>GSELRSIAFSRAVFAEFLATLLFVFFGLGSALNWPQALPSVLQIAMAFGLGIGTLVQALGHISGAHINPAVTVACLVGCHVSVLRAAFYVAAQLLGAVAGAALLHEITPADIRGDLAVNALSNSMTAGQAVTVELFLTLQLVLCIFASTDERRGENPGTPALSIGFSVALGHLLGIHYTGCSMNPARSLAPAVVTGKFDDHWVFWIGPLVGAILGSLLYNYVLFPPAKSLSERLAVLKGLE[4x]

Aquaporins are water channels found in the cell membrane, where they allow the passage of water molecules in and out of the cells. In the kidney collecting duct, arginine vasopressin-dependent trafficking of aquaporin-2 (AQP2) fine-tunes reabsorption of water from pre-urine, allowing precise regulation of the final urine volume. Point mutations in the gene for AQP2 may disturb this process and lead to nephrogenic diabetes insipidus (NDI), whereby patients void large volumes of highly hypo-osmotic urine. Here we describe the structural and functional characterization of three AQP2 mutations associated with recessive NDI: T125M and T126M, situated close to a glycosylation site and A147T in the transmembrane region.

T125M and T126M are located in extracellular loop C, immediately downstream to an N-glycosylation site at Asn 123. T125M is located within the glycosylation consensus sequence (Asn-X-Ser/Thr) and this mutant can therefore not be glycosylated. Consequently, T125M is absent from the plasma membrane when expressed in oocytes. It seems plausible that, similar to N123Q, also this mutant is kept in the Golgi, after which it may be degraded via ESCRT-dependent targeting to lysosomes or the more recently identified Endosome and Golgi-associated degradation (EGAD) pathway. Overall, T126M gave crystals which diffracted to highest resolution, (~3–3.3 Å), followed by T125M (~3.7–4 Å). The T125M and T126M-structures are highly similar to wild-type AQP2, with root-mean-square deviations (RMSD) of 0.942 Å (929 Cα-atoms) for T125M and 0.322 (940 Cα-atoms) for T126M. In the T125M structure, a minor displacement of the main chain could be observed around Asn 123 and Ser 124 (1–2 Å), most likely due to the larger methionine side chain. It thus seems that AQP2 can accommodate the replacement of a small polar residue with a larger hydrophobic one without any significant structural rearrangements. It should be mentioned that, in particular for T125M, the resolution is not high enough to reliably obtain information about interactions between residues and that there may be minor structural alterations regarding side-chain conformations and hydrogen bonds that we are not able to ascertain.NITROISOCITRIC ACID 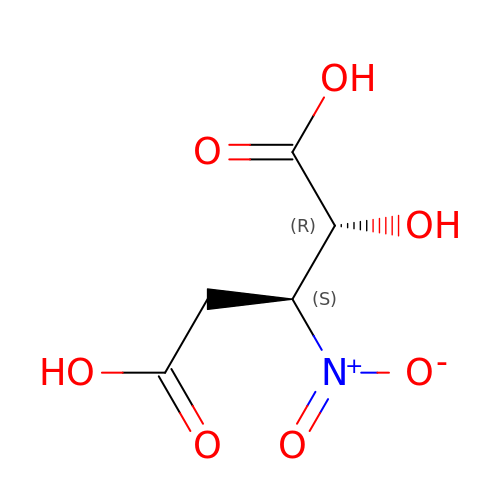| C5 H7 N O7 | ZTJSGPUFCRRTOT-ZAFYKAAXSA-N LOV-HK is a blue light photoreceptor from Brucella abortus, a pathogenic α-2-proteobacterium that can be transmitted from cattle to humans causing brucellosis. B. abortus LOV-HK comprises an N-terminal blue light-sensing LOV domain, a central PAS (Per-Arnt-Sim) domain of unknown function and a C-terminal HK domain. The LOV and PAS domains are connected through a long linker helix denoted the Jα helix, while the HK domain belongs to the HWE family. Upon blue light illumination, B. abortus LOV-HK photobleaches as a result of the adduct formation between its flavin mononucleotide (FMN) chromophore and an adjacent conserved cysteine residue as in other LOV proteins.

We have determined the crystal structure of LOV-PAS in the dark-adapted state at 2.74 Å resolution. The chromophore environment in the LOV-PAS structure is consistent with the dark structures of B. abortus LOV domains and other LOV proteins, where the FMN ligand is clearly separated from the protein moiety in the electron density map (left). In the asymmetric unit, four LOV-PAS polypeptide chains form two elongated parallel dimers. In each dimer, the LOV domains, the linker helices, and the PAS domains from the partner subunits are juxtaposed along the extensive dimer interface. The tandem LOV and PAS domains from the same subunit have no direct contact, and their dispositions are swapped relative to the helical spine resulting in a cross-shaped dimer. At the dimer interface, two long Jα helices (residues 135 to 171) consisting of five heptad repeats form an extensive coiled coil via mainly hydrophobic interactions. Although the LOV-PAS structure is rather straight, modest dimer asymmetry is evident when the four monomers present in the asymmetric unit are aligned according to the LOV domain. The CD dimer exhibits slightly higher asymmetry than the AB dimer. In the dark LOV structure, the isoalloxazine moiety of FMN forms extensive H-bonds with the conserved Asn101/Asn111 and Gln132 residues, while its phosphate group extends out between the Eα and Fα helices.

>MALSQATDPFRAAVEFTLMPMLITNPHLPDNPIVFANPAFLKLTGYEADEVMGRNCRFLQGHGTDPAHVRAIKSAIAAEKPIDIDIINYKKSGEAFWNRLHISPVHNANGRLQHFVSSQLDVTLELSRLVELEKERKTLSIETARSKDQLDYIVEVANIGFWTREFYSGKMTCSAECRRIYGFTPDEPVHFDTILDLVVLEDRMTVVQKAHQAVTGEPYSIEYRIVTRLGETRWLETRAKALTGENPLVLGIVQDVTERKHHHHHH[4x]Aconitase superfamily members catalyze the homologous isomerization of specific substrates by sequential dehydration and hydration and contain a [4Fe-4S] cluster. However, monomeric and heterodimeric types of function unknown aconitase X (AcnX) have recently been characterized as a cis-3-hydroxy-L-proline dehydratase (AcnXType-I) and mevalonate 5-phosphate dehydratase (AcnXType-II), respectively. We herein elucidated the crystal structures of AcnXType-I from Agrobacterium tumefaciens (AtAcnX) and AcnXType-II from Thermococcus kodakarensis (TkAcnX) without a ligand and in complex with substrates. AtAcnX and TkAcnX contained the [2Fe-2S] and [3Fe-4S] clusters, respectively, conforming to UV and EPR spectroscopy analyses.

Ser70 in AtAcnX may be sequentially homologous to Ser642 in mAcn, which functions as a general base; the purified S70A mutant is almost inactive and brown in color, similar to the wild-type enzyme. Therefore, to obtain a more-detailed understanding of substrate binding, we elucidated the crystal structure of the S70A mutant of AtAcnX in complex with C3LHyp at a resolution of 2.0 Å using a co-crystallizing method; this structure had a similar conformation to that of the wild-type enzyme in the apo-form, with an r.m.s.d. value of 0.4 Å for 559 Cα atoms. This mutant enzyme had the same [2Fe-2S] cluster as the wild-type enzyme, and additional electron density around the [2Fe-2S] cluster was clearly modeled as C3LHyp. The carboxyl group of bound C3LHyp formed hydrogen bond(s) and/or salt bridge(s) with a water molecule (Wat16), the side chains of Ser293 and Lys530, and the main chain nitrogen atoms of Cys71 and Ser293. The nitrogen atom of C3LHyp made a hydrogen bond and/or salt bridge with the side chains of Thr72 and Asp203, respectively. The C3-OH group interacted with the Fe1 atom and side chains of Glu292 and Lys530. The hydrophobic side chains of Trp35 and Ile206 interacted with the C4-C5 backbone of the pyrrolidine ring of C3LHyp, which may explain the extremely poor utilization of 2,3-cis-3,4-cis-3,4-dihydroxy-l-proline (C3LHyp with the additional hydroxyl group on C4) as a substrate. Ser70 was clearly the first candidate as a general base because when the structure of the apo-form of the wild type was superimposed onto that of the holo-form of the S70A mutant, the side chain of Ser70 was close to C2 of C3LHyp (a distance of 2.7 Å). Therefore, we propose that the dehydration reaction begins by the abstraction of a proton from C2 of C3LHyp by the alkoxide form of the Ser70 side chain, similar to mAcn (Ser642). The Fe2 atom, which exists in the [2Fe-2S] cluster in the Fe3+ oxidation state, acts as a Lewis acid that accepts the electron pair from the leaving hydroxyl group on C3.

>[4x]MRGSHHHHHHGSSAVSTTAAPEARSILAGAAEGKVIATTEALSFWGGVDPATGKVIDVHHPLHGICLTGGVLFMPTSRGACTGSGVLLDLILTGRAPSALVFCEAEDVLTLGALVAAEMFDKALPVIRLDTETFARFSRAAHVRIDQNTIKADGVSLAVAPPATAHLDLTDDDRAMLEGRDGIAVRQAMRIIVAMAAQQGASALVDVTQGHIDGCIYASPANLTFAEKMADMGGKVRVPSTMNAISVDKANWRAQGVPEDFGDPAARLADAYVRMGCRPTFTCSPYLLDSAPSAGESIGWAESNAVIFANTVLGARTAKHPDFLDLCIAMTGRAPLSGVYLEENRRPQRIVDVALPAGIDDAFWPLVGYLAGKAVPDCIPLLRGLGAAKPSRDDLKALCAAFGTTSASPMLHIEGATPEAGLAPLETAETVTISLEDMAAGWSLLNEGPEEVQLVAIGSPHASLEECRALAAVFNGRKRHADVAVIVTAGQQVIDAAGKDGTLQSLKDSGVQVLPDLCWCSISEPVFPTKTRALMTNSGKYAHYGPGLSGRAVRFGSLADCVESALTGRAVSRLPVWLS>GAGTVASVAGTATASGIASGTVNLVGGGQVKNIAIAAGDSAKAIAEKMDGAIPNLSARARTVFTADVSGVTGGSLNFDVTVGSNTVSLAGVTSTQDLADQLNSNSSKLGITASINDKGVLTITSATGENVKFGAQTGTATAGQVAVKVQGSDGKFEAAAKNVVAAGTAATTTIVTGYVQLNSPTAYSVSGTGTQASQVFGNASAAQKSSVASVDISTA[2x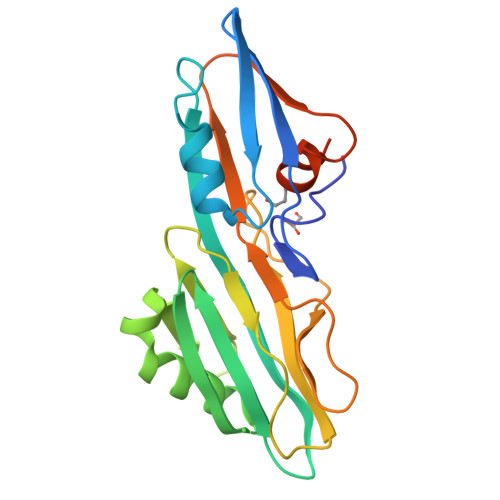]> MHPMLNIAVRAARKAGNLIAKNYETPDAVEASQKGSNDFVTNVDKAAEAVIIDTIRKSYPQHTIITEESGELEGTDQDVQWVIDPLDGTTNFIKRLPHFAVSIAVRIKGRTEVAVVYDPMRNELFTATRGQGAQLNGYRLRGSTAR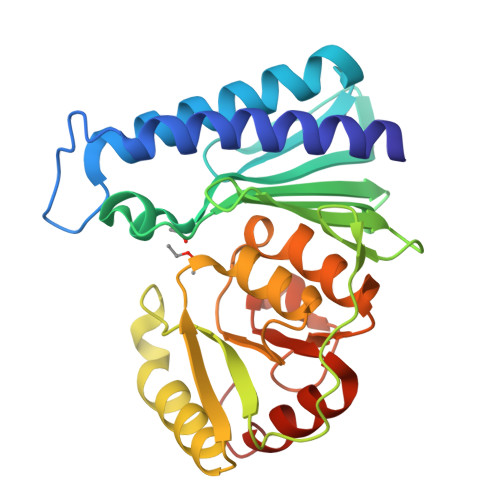DLDGTILATGFPFKAKQYATTYINIVGKLFNECADFRATGSAALDLAYVAAGRVDGFFEIGLRPWDFAAGELLVREAGGIVSDFTGGHNYMLTGNIVAGNPRVVKAMLANMRDELSDALKR> MAHMVNGKVALVTGAAQGIGRAFAEALLLKGAKVALVDWNLEAGVQCKAALHEQFEPQKTLFIQCDVADQQQLRDTFRKVVDHFGRLDILVNNAGVNNEKNWEKTLQINLVSVISGTYLGLDYMSKQNGGEGGIIINMSSLAGLMPVAQQPVYCASKHGIVGFTRSAALAANLMNSGVRLNAICPGFVNTAILESIEKEENMGQYIEYKDHIKDMIKYYGILDPPLIANGLITLIEDDALNGAIMKITTSKGIHFQDYGSKENLYFQ

15-hydroxyprostaglandin dehydrogenase (15-PGDH, EC 1.1.1.141) is the key enzyme for the inactivation of prostaglandins, regulating processes such as inflammation or proliferation. 15-PGDH represents the key enzyme in the inactivation of a number of active prostaglandins, leukotrienes and hydroxyeicosatetraenoic acids (HETEs) (e.g., by catalyzing oxidation of PGE2 to 15-keto-prostaglandin E2, (15k-PGE)). Human type-I 15-PGDH is encoded by the HPGD gene and belongs to the evolutionarily conserved superfamily of short-chain dehydrogenase/reductase enzymes (SDRs), within which it is classified as SDR36C1. The enzyme has been purified from human placenta and its primary structure determined by Edman degradation; it was subsequently cloned and characterized as a homodimer with subunits of a size of 29 kDa.

After several unsuccessful crystallization attempts with constructs bearing different tags fused to the N- or C-terminus, respectively, it was possible to grow crystals in presence of NADH from a construct purified with a C-terminal His6 tag and to determine for the first time the structure of the homodimer of 15-PGDH in a complex with its cofactor at a resolution of 1.65 Å. This resolution is not high enough to distinguish the reduced state of the cofactor from its oxidized form. The protein shows the α/β folding pattern that is highly conserved among the short-chain dehydrogenases/reductases (SDR), where a central β-sheet consisting of 8 strands is flanked on either side by two arrays of α-helices (Rossmann fold). In the crystallized construct the last ten amino acids from the 15-PGDH sequence are missing, leaving Tyr256 as the last native amino acid. Instead, the cloning procedure resulted in the fusion of nine non-natural amino acids (Gly-Ser-Lys-Glu-Asn-Leu-Tyr-Phe-Gln) to the C-terminus remaining after cleavage of the tag. In the structure of the dimer the artificial C-terminus of one protomer is folded over the top of the opposing protomer (highlighted in orange in Figure 5), with a number of residues engaging in interactions with side chains of the other protomer, notably between Phe264 and Tyr217. The acidic residue Asp36 forms hydrogen bonds to the 2′- and 3′-hydroxyl groups of the adenine ribose moiety, while Asp64 forms a hydrogen bond to the amino group of the adenine moiety. The nicotinamide moiety of NAD+ is positioned close to the catalytic tetrad (Asn107, Ser138, Tyr151 and Lys155), competent for the hydride transfer from the S-side of C4 to the substrate following the reaction mechanism conserved among all SDRs.>X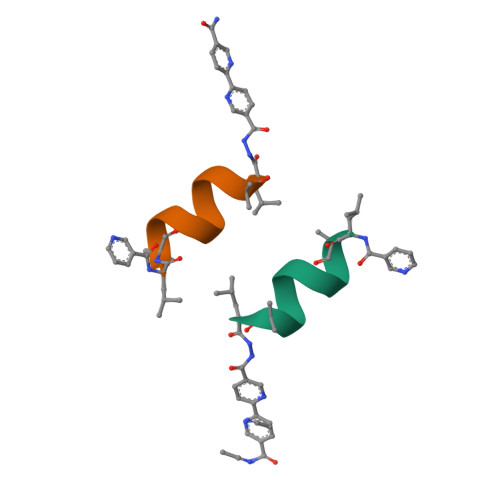LAACLCCALX[2x]> MGSVNSSPNEEFETVPDSQISGFDSPLIPTSVGSYFRDDDDDEKVHPNFISDPENDSLNSDEEFSSLENSDLNLSGAKAESGDDFDPILKRTIISKRKAPSNNEDEEIVKTPRKLVNYVPLKIFNLGDSFDDTITTTVAKLQDLKKEILDSPRSNKSIVITSNTVAKSELQKSIKFSGSIPEIYLDVVTKETISDKYKDWHFISKNCHYEQLMDLEMKDTAYSFLFGSSRSQGKVPEFVH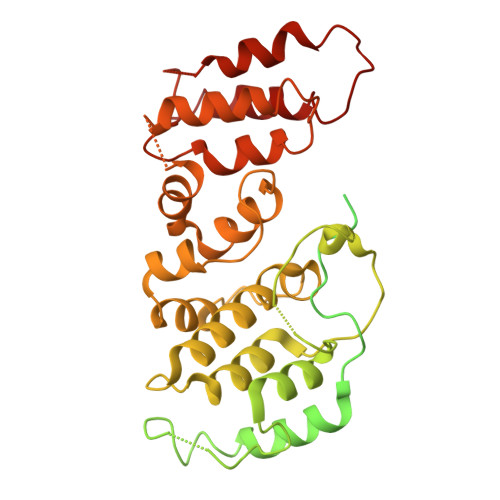LKCPSITNLLVLFGVNQEKCNSLKINYEKKENSRYDNLCTIFPVNKMLKFLMYFYSDDDNDDVREFFLKAFICLILDRKVFNAMESDHRLCFKVLELFNEAHFINSYFEIVDKNDFFLHYRLLQIFPHLQSALLRRRFSEKQGRTETIQQNIIKEFNEFFDCKNYKNLLYFILTMYGSKFIPFGPKCQVTEYFKDCILDISNETTNDVEISILKGILNLFSKIR>[2x]DIPQQLVERLQEEKRIEAQKRKERQEAHLYMQVQIVAEDQFCGHQGNDMYDEEKVKYTVFKVLKNSSLAEFVQSLSQTMGFPQDQIRLWPMQARSNGTKRPAMLDNEADGNKTMIELSDNENPWTIFLETVDPELAASGATLPKFDKDHDVMLFLKMYDPKTRSLNYCGHIYTPISCKIRDLLPVMCDRAGFIQDTSLILYEEVKPNLTERIQDYDVSLDKALDELM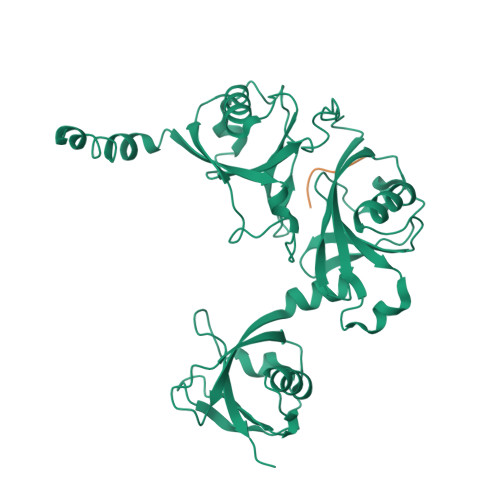DGDIIVFQKDDPENDNSELPTAKEYFRDLYHRVDVIFCDKTIPNDPGFVVTLSNRMNYFQVAKTVAQRLNTDPMLLQFFKSQGYRDGPGNPLRHNYEGTLRDLLQFFKPRQPKKLYYQQLKMKITDFEN;> PRKKKRKH4-(6-azanyl-8-bromanyl-purin-9-yl)butan-1-ol | C9 H12 Br N5 O | 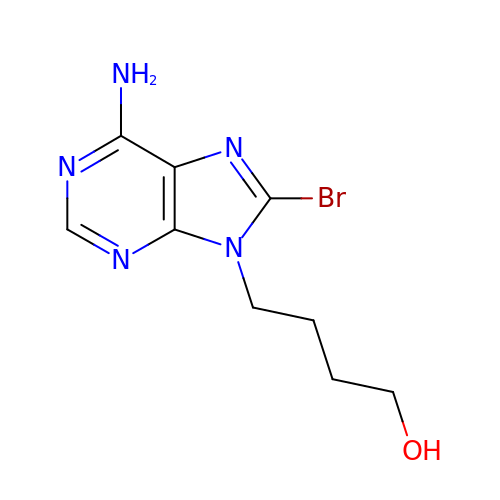XPHFIISDJKTZOQ-UHFFFAOYSA-N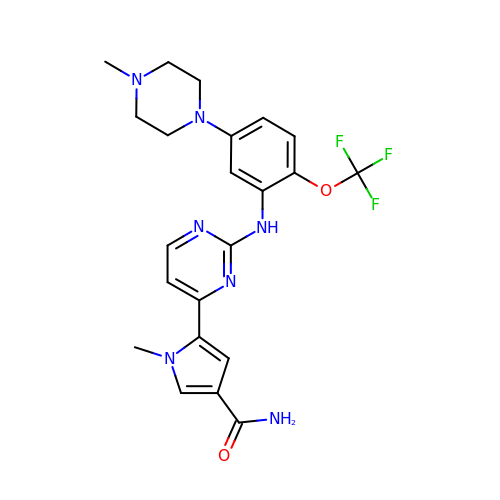1-METHYL-5-(2-{[5-(4-METHYLPIPERAZIN-1-YL)-2-(TRIFLUOROMETHOXY)PHENYL]AMINO}PYRIMIDIN-4-YL)-1H-PYRROLE-3-CARBOXAMIDE | C22 H24 F3 N7 O2 | HGBZKLOZYQAERY-UHFFFAOYSA-N> GVKSLKRRRC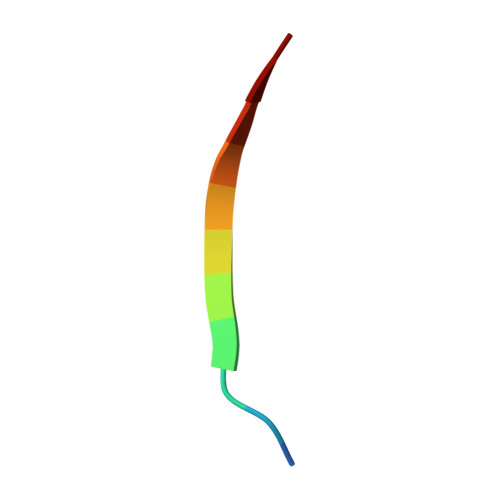Y>[2x]GMQNSQEMAITTLSLPKGGGAINGMGESVGQAGPDGMVTFSIPLPFSAGRGVAPALSLSYSSGAGNGPFGMGWQCSAMSISRRTQKGVPQYNEDDEFLSPSGEVMAIALNDSGFEDVRTANRLQGIPLPFSYKVTRYQPRLIQDFIKIEYWQPVKQTDGTPFWIIYSPDGQTHILGKNSHSRVANAENPSQIASWLLEETVTPTGEHIYYQYSGENQVNCTDAEIALHPQDSAQRYLARIDYGNISPQASLFVLDEELPNLTQWLFHLVFDYGERDISINKIPTFEGGTTGWLARPDMFSRYDFGIEIRNRRLCHQVLGFHRLEALNDRDVTDEIPVLVNRLTLDYDLNNSVSTLVAVRQVAYETDGSPITQPPLEFDYQRFDTGSIPGWQEMPQLEAFNGYQPYQMIDLYGEGTPGILYQETPGAWWYKSPQRQIGGDSNAVTYGAMKALPKIPRLQEGATLMDINGDGRLDWVITSAGVRGFHSIHSTGEWTHFTPLNTLPTEYFHPKAQLADLVGAGLSDLVLIGPKSVRLYANQQGNWAPAQDVTQAENVSLPVIGIDSRQLVAFADMLGSGQQHLVEITADSVKCWPNMGHGRFGQPLTLEGFSQPQTSFNPDRVFLADIDGSGTNDIIYAHSECLEIYLNESGNRFSKPISLLLPDGVNFDNTCQLQAADIQGLGIASLVMTVPHMSPTHWRCDLALNKPWLLNVMNNNRGAETCLFYRSSAQFWLDEKQLVEAAGQQPECHLPFPMHLHWRSEIFDEITGNRLTQEQEYAHGSWDGQEREFRGFGRLIQRDTDGFAQGTVDIPTHPSRTVSWFATGIPEIDTTLSAEFWRGDDQAFSPFSPRFTRWENDSEAGSDVAFIPSEHDAFWLNRAMKGQLLRSELYGDDGTPEAEIPYSVTEMRHQVRALPTTDATVPSAWCSTIETRSYQYQRVAADPQCSQQVVIKADRYGSPLLSVAINYPRRKKPEKSPYPDDLPETLFDSSYDTQQQQLHLTKQQQNYFHLTNDDNWLLGLPKEQRNDGYQYDQERAPANGFTLETLIASNSLIGSNQPFTYLGQSRVAYQGGVDEQPSLQALVAYGETAILDEKTLQAFVGVLDSKTRDELLFSAG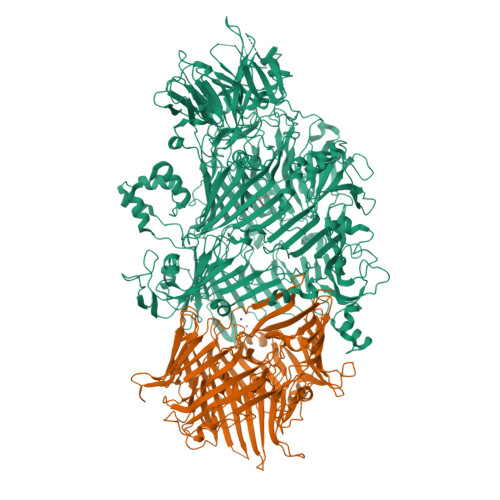YQLAPRLFRVESEPDVWVARQGYSEFGDYSQFWRPLSQRSTLLTGKTTLKWDKHYCVVIETQDAAQLVTQARYDYRFLTPYSLTDANDNQHYVVLNPFGEVIASRFWGTEAGKDAGYSTPQAKPFVVPATIEAALALSPGIPVAHCAIFEPESWMQKLTQHDVSERMADNGTLWNALLQARFVTEDGYVCALGRRRWMARHGLSVLMLTLLAEIPRTPPHSLTITTDRYDSDDQQQLRQRILFSDGFGRLLQSAQRVEAGESWQRSEDSSLVVNVSGTPALVVTDNRWAVSGRTEYDGKGQGIRVYQPYFLDDWRYLSDDSARTDLFADTHIYDPLGREYQVITAKGYRRERQYTPWFVVNQDENDTAANLAI;>MDIQLFSKTPSVTVFDNRGLSVRDIAYRRHPDTPKVTEECITYHQFDFRGFLAQSLDPRLNHKEVTNFSYLTDLNGNIIYTQSVDAGNTLVLNDTEGRSVIAMTNISRGENGKDDLSLAVTRTFQYENAPLPGRPLSVTEQVNGENARITEHFVYAGNTPQEKNLNLAGQCVSYYDAAGLIQTDSVSLTGKPLSVSRKLLKNLDDTNILADWQGNDTSAWNSLLATEIYTTVTRTDAAGAVLTTIDAVGNQQRVAFDIAGQLSASWLTLKGGQEQVIIKVLTYSAAGQKLREEGGNGVVTTYTYEAETQRLIGIKTERPNGHAAGAKVLQDLRYEYDPVGNVLSITNDAEETRFWRNQKVVPENAYRYDSLYQLVSASGREVAGAGQQGSDLPSPLVPLPSDSSVYTNYTRTYTYDSAGNLMRIRHSAPATNNNYTLNITVSERSNRGVMSSLTENPADVDALFTASGSQKCLQQGQSLIWTPRGELRTVLLVARGETADDSESYRYDGSSQRILKISSQQTNHSARVQRALYLPGLEWRTMTGGVAEAENLQVICIGEAGRAQVRVLHWESGKPDGIINDQIRWSYDNLTCSSGLEVDGDGLVISMEEYYPYGGTAVWAARSHIETAYKTVRYSGKERDATGLYYYGFRYYQPWAGRWLSADPAGTVDGLNLYRMVRNNPLRLTDPDGM[2x]> GYIQGTHVKTDLPGPFHITMSPDGSTLFISNQSGHSVTFVDARTQKVTGEVAVRVQPEASAVTPDGAFLYVCNAESDSVSVVDIQRKQEIKEIKVGDWPSGIKISPDGKTAYVACSGCMW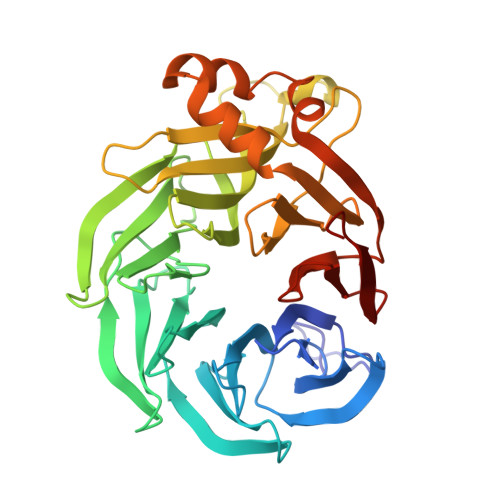NAIDVIDTGRMEKVRSIYTSDYGPRMVEISPDGKTLVAILDTVGSINRSVDFIDIASGRVVENRVIHESSNLRDVVYTPDGKYIAVTHQTPKNWLPVCEAENGQVFTNNVTIIETKAGGKVARLPLDDLNNYDGNPYGMAMDPKGKYLYIGVRGMHRVTILDMDKVLGLVRSSTQEELDYLRDDLGLVRDYLVARVPTGLGPSSVCLSPDGKFCYAANYFSNNVTVIRTAVD> SQQDG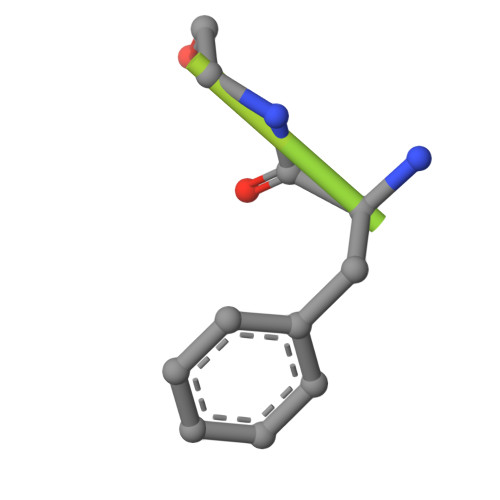SLRSRKANLETGAFGKSTRRTRSKAATPAKRED>GPMNIINTSILNLRYESNHLIDLSRYASKINIGSKVNFDPIDKNQIQLFNLESSKIEVILKNAIVYNSMYENFSTSFWIRIPKYFNSISLNNEYTIINCMENNSGWKVSLNYGEII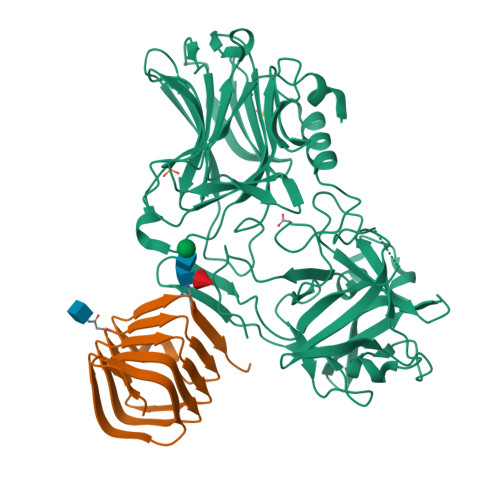WTLQDTQEIKQRVVFKYSQMINISDYINRWIFVTITNNRLNNSKIYINGRLIDQKPISNLGNIHASNNIMFKLDGCRDTHRYIWIKYFNLFDKELNEKEIKDLYDNQSNSGILKDFWGDYLQYDKPYYMLNLYDPNKYVDVNNVGIRGYMYLKGPRGSVMTTNIYLNSSLYRGAKFIIKKYASGNKDNIVRNNDRVYINVVVKNKEYRLATNASQAGVEKILSALEIPDVGNLSQVVVMKSKNDQGITNKCKMNLQDNNGNDIGFIGFHQFNNIAKLVASNWYNRQIERSSRTLGCSWEFIPVDDGWGERPL[2x];>SHHHHHHHHHSGGGSGGGIEGRVERDKYANFTINFTMENQIHTGMEYDNGRFIGVKFKSVTFKDSVFKSCTFEDVTSVNTYFKNCTFIDTVFDNTDFEPYKFIDSEFKNCSFFHNKT[2x]> MTQTQPVTPTPPASFQTQHDPRTRLGATPLPGGAGTRFRLWTSTARTVAVRVNGTEHVMTSLGGGIYELELPVGPGARYLFVLDGVPTPDPYARFLPDGVHGEAEVVDFGTFDWTDADWHGIKLADCVFYEVHVGTFTPEGTYRAAAEKLPYLKELGVTAI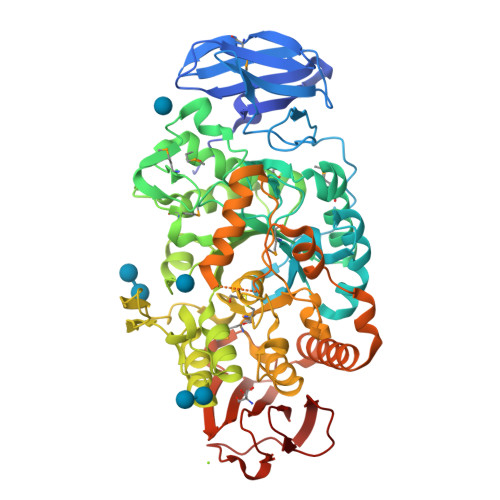QVMPLAAFDGQRGWGYDGAAFYAPYAPYGRPEDLMALVDAAHRLGLGVFLDVVYNHFGPSGNYLSSYAPSYFTDRFSSAWGMGLDYAEPHMRRYVTGNARMWLRDYHFDGLRLDATPYMTDDSETHILTELAQEIHELGGTHLLLAEDHRNLPDLVTVNHLDGIWTDDFHHETRVTLTGEQEGYYAGYRGGAEALAYTIRRGWRYEGQFWAVKGEEHERGHPSDALEAPNFVYCIQNHDQIGNRPLGERLHQSDGVTLHEYRGAAALLLTLPMTPLLFQGQEWAASTPFQFFSDHAGELGQAVSEGRKKEFGGFSGFSGEDVPDPQAEQTFLNSKLNWAEREGGEHARTLRLYRDLLRLRREDPVLHNRQRENLTTGHDGDVLWVRTVTGAGERVLLWNLGQDTRAVAEVKLPFTVPRRLLLHTEGREDLTLGAGEAVLVG N-methyl-2-thiophenesulfonamide 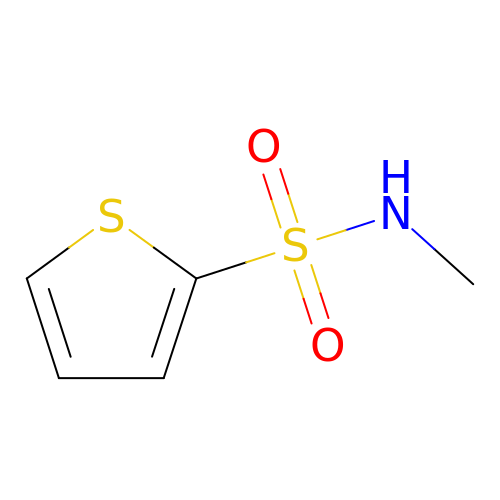| C5 H7 N O2 S2 | CTIGHRXLNNYNGU-UHFFFAOYSA-N> KPQIPKDKSKVAGYIEIPDADIKEPVYPGPATPEQLNRGVSFAEENESLDDQNISIAGHTFIDRPNYQFTNLKAAKKGSMVYFKVGNETRKYKMTSIRDVKPTDVGVLDEQ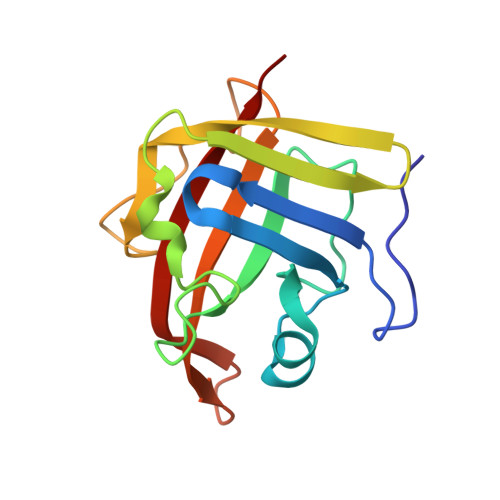KGKDKQLTLITADDYNEKTGVWEKRKIFVATEVK>[2x]HHHHHHQPVEQLSFDELTLINLSKVVTVNGHEVPMRIKEFELLWYLASRENE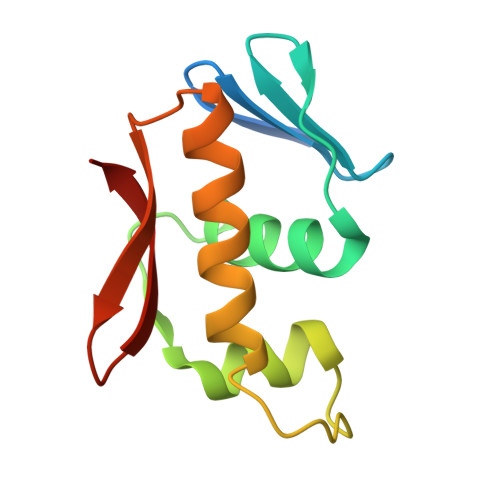VISKSELLEKVWGYDYYEDANTVNVHIHRIREKLEKESFTTYTITTVWGLGYKFERSR>[2x]MALVDGFLELERSSGKLEWSAILQKMASDLGFSKILFGLLPKDSQDYENAFIVGNYPAAWREHYDRAGYARVDPTVSHCTQSVLPIFWEPSIYQTRKQHEFFEEASAAGL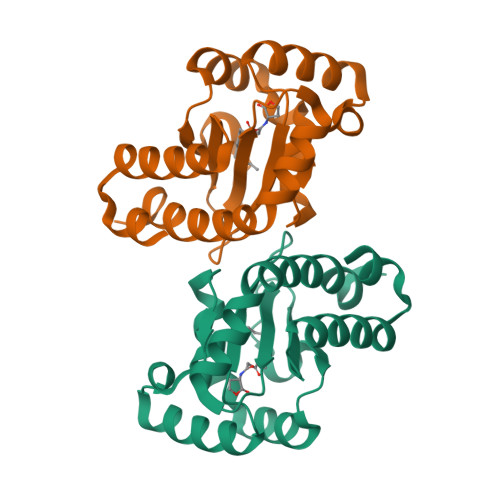VYGLTMPLHGARGELGALSLSVEAENRAEANRFMESVLPTLWMLKDYALQSGAGLAFEHPVSK> M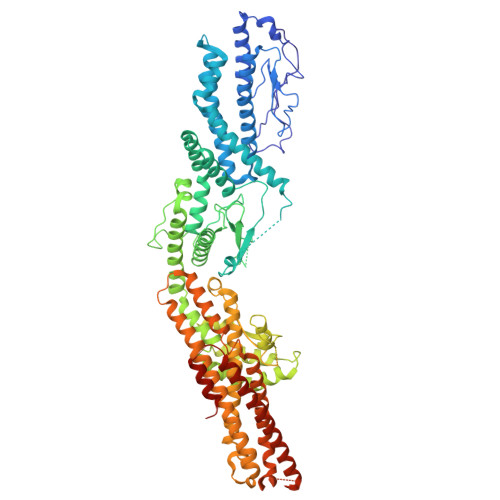EIKEVDDRAELLRYTNNIPLLGKLVNHQPLWSTNPKLKSFSLEKISAPDQRRVQEALVVKDLLNVLIGLEGTYIRYFNDYEPSDPETPIEFKIAKKMDPSFKTFSRRIVRYGKQYMILTRAYEKWSDTSFGMVLQRFAYEIRRFLEDVYLKTLVERLERDFNKVPNFSIRELEQIINETEVNKQMELLYNIYEEIFREIEERRTNQSSQEDFNNFMDSMKNESSLHLRLMVAFDTTVYPVPKGGAILKIFQQKILENLGDRSSVMFLKKLLNNISQDYCTMLYEWLTQGILNDPYQEFMTYDDLEGKTDNIFDTRDRAWDTQYFIRKDVLLRDCDSEEDKNLLFKMLRTGILLKVVRASLQIPTIPSNSSDITIQEINDFADLMEGSNLELYVDKCYSRANEIFLKLFFQGYDLINVLKHLQQIFLGYQSGHNVLKFLTKNMGELTKHYRNDNNANYDKLLQNFELERQSENPNNLMRQLLMIQFDTETLPQVLSHYLQIYPEVPENNSANDDSDPLMHANNFKNMNAILFDELSKERTGAYHGSNLELYTPKSAIYHLKFDINIPYPLNIIISRTCMIKYQIILRYQLVLQYHSRLLDETWMDLNKTPSWKYRGYSHTVKRRIVRATRVLHAKMNHFIKTIMEYFNQNVIDKEVYSLEKCYRNPTLAVAIQNELEGGLTNIMTNRCLSDLIPLQLQIFDIVYKFCKFIKSMRAKLCQLDPVLYEKHKSGMMKTLNEGYRTNNGGQEDVGYQEDAALELIQKLIEYISNASSIFRKCLINFTQELSTEKFDFYDSSSVDAAGIERVLYSIVPPRSASASSQR> GSFGFGVPAAPVLPFGLTPKKVYKPEVQLRRPNWSKFVAEDLSQDCFWTKVKEDRFENNELFAKLTLAFSAQTKTSKAKKDQEGGEEKKSVQKKKVKELKVLDSKTAQNLSIFLGSFRMPYQEIKNVILEVNEAVLTESMIQNLIKQMPEPEQLKMLSELKEEYDDLAESEQFGV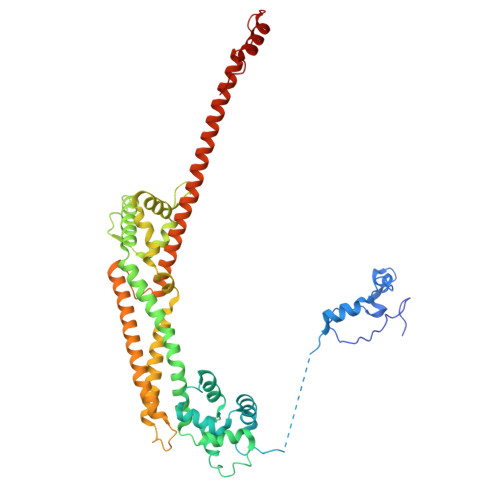VMGTVPRLRPRLNAILFKLQFSEQVENIKPEIVSVTAACEELRKSENFSSLLELTLLVGNYMNAGSRNAGAFGFNISFLCKLRDTKSADQKMTLLHFLAELCENDHPEVLKFPDELAHVEKASRVSAENLQKSLDQMKKQIADVERDVQNFPAATDEKDKFVEKMTSFVKDAQEQYNKLRMMHSNMETLYKELGDYFVFDPKKLSVEEFFMDLHNFRNMFLQAVKENQKRRETEEKMRRAKLAKEKAEKERLEKQQKREQLIDMNAEGDETGVMDSLLEALQSGAAFRRKRG> WMDFD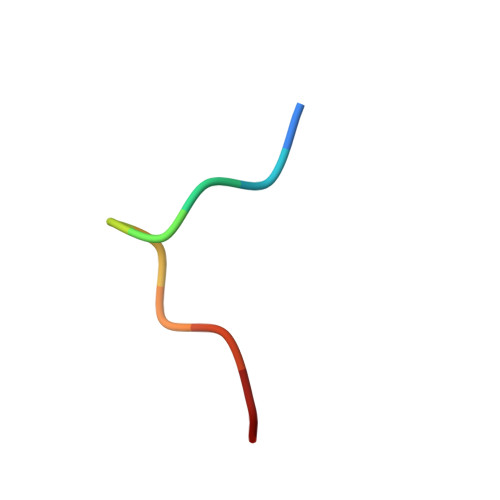DDIPF>GGADQKGPVFLKEPTNRIDFSNSTGAEIECKASGNPMPEIIWIRSDGTAVGDVPGLRQISSDGKLVFPPFRAEDYRQEVHAQVYACLARNQFGSIISRDVHVRAVVQQFYESEVNNEYVIRGNAAVLKCSIPSFVADFVQVVSWQDEEGQLYGSLGDQQGTDGKYLVLPSGELHIREVGPEDGYKSYQCRTKHRLTGETRLSATKGRLVITEPVGSKAPTFATASKISSLLGSSSSDIVLLCQAQAFPVPYTRWYKFIEGTTRKQAVVLNDRVKQVSGTLIIKDAVVEDSGKYLCVVNNSVGGESVETVLTVTAPLSAKIDPPTQTVDFGRPAVF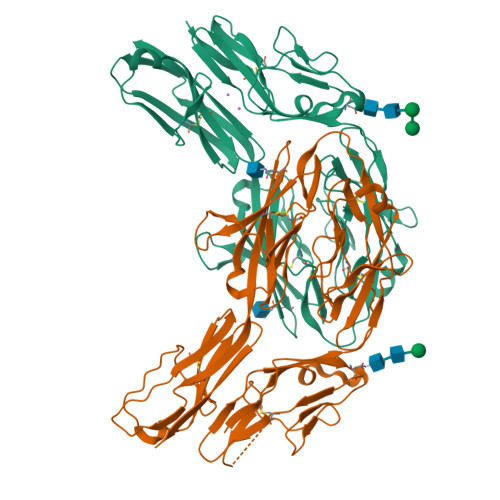TCQYTGNPIKTVSWMKDGKAIGHSEPVLRIESVKKEDKGMYQCFVRNDQESAEASAELKLGG[2x]> MNHKVHHHHHHIEGRHMKRLTYISKFSRPLSGDEIEAIGRISSQKNQQANVTGVLLCLDGIFFQILEGEAEKIDRIYERILADERHTDILCLKSEVEVQERMFPDWSMQTINLDENTDFLIRPIKVLLQTLTESHRILEKYTQPSIFKIISQGTNPLNIRPKAVEKIVFFSDIVSFSTFAEKLPVEEVVSVVNSYFSVCTAI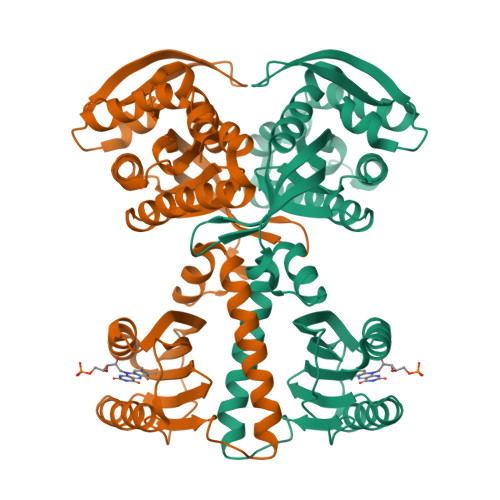ITRQGGEVTKFIGDCVMAYFDGDCADQAIQASLDILMELEILRNSAPEGSPLRVLYSGIGLAKGKVIEGNIGSELKRDYTILGDAVNVAARLEALTRQLSQALVFSSEVKNSATKSWNFIWLTDSELKGKSESIDIYSIDNEMTRKSSGGLEIARNIGHYLERVGDRQPSQIFGVKSLPL> MHVVYPGSFDPLTNGHLDVIQRASRLFEKVTVAVLENPSKRGQYLFSAEERLAIIREATAHLANVEAATFSGLLVDFVRRVGAQAIVKGLRAVSDYEYELQMAHLNRQLYPGLETLFILAATRYSFVSSTMVKEIARYGGDVSKL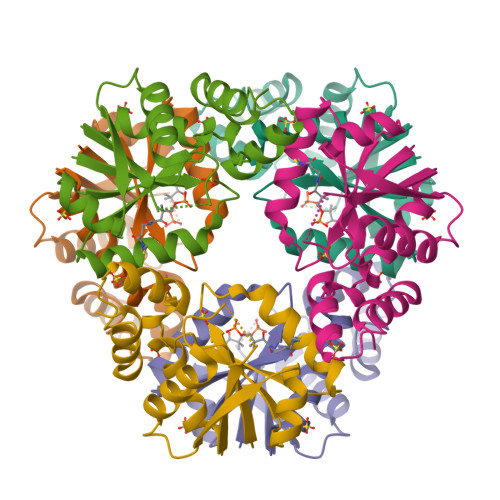VPPATLRALKAKLGQ> MTRLLVLGGTTEASRLAKTLADQGFE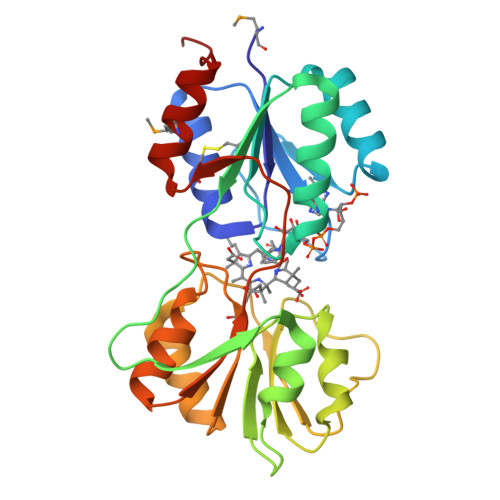AVFSYAGRTGAPVAQPLPTRIGGFGGVAGLVDYLTREGVSHVIDATHPFAAQMSANAVAACAQTGVALCAFERAPWTAQAGDRWTHVPDLAAAVAALPQAPARVFLAIGKQHLRDFSAAPQHHYLLRLVDPPEGPLPLPDARAVIARGPFTVQGDTELLRSETITHVVAKNAGGAGAEAKLIAARSLGLPVILIDRPAVPARDICATLEGVMGWLADHGATPRGV> GLPV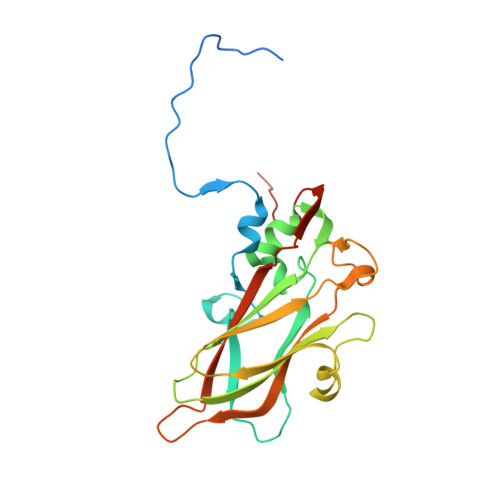MLTPGSGQFLTTDDTQSPSAFPYFHPTKEIFIPGQVRNLIEMCQVDTLIPVNNTQENVRSVNMYTVDLRTQVDLAKEVFSIPVDIASQPLATTLIGELASYYTHWTGSLRFSFMFCGSASSTLKLLIAYTPPGVGKPKSRREAMLGTHLVWDVGLQSTASLVVPWVSASHFRFTTPDTYSSAGYITCWYQTNFVVPDSTPDNAKMVCMVSACKDFCLRLARDTNLHTQEGVLTQ>GAMSEAFHTHSGIGVPLRRSNVDTDQIIPAVFLKRVTRTGFEDGLFAGWRSDPAFVLNLSPFDRGSVLVAGPDFGTGSSREHAVWALMDYGFRVVISSRFGDIFRGNAGKAGLLAAEVAQDDVEILWKLIEQSPGLEITANLQDRIIT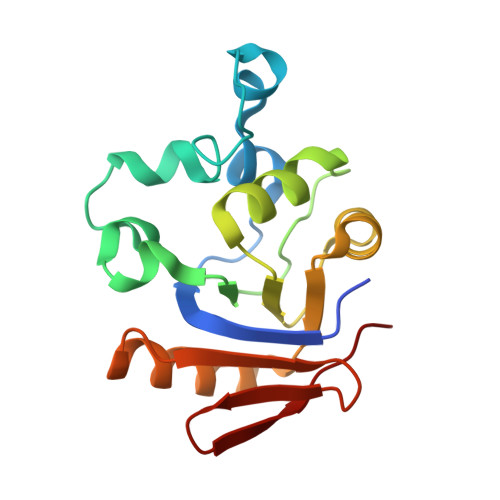AATVVLPFKID[2x]> DDSVLA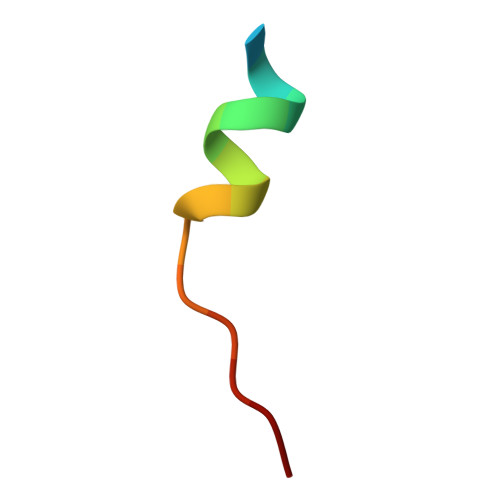ARARMWMWHW>[4x]MQWSGARALEALLTVAGELRGPPLQLDTGQLLKIAKRGGVTAVEAVHAWRNALTGAPLNLTPEQVVAIASHDGGKQALETVQRLLPVLCQAHGLTPQQVVAIASHDGGKQALETVQRLLPVLCQAHGL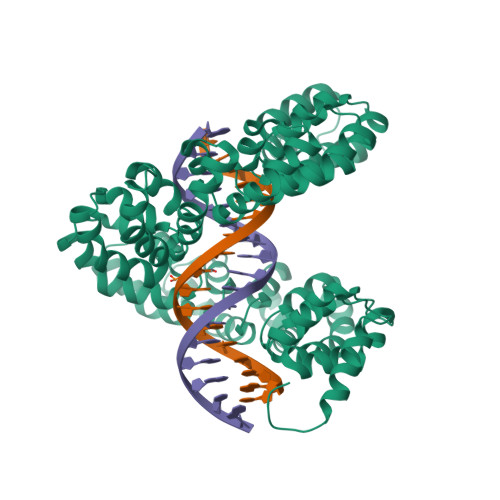TPEQVVAIASHDGGKQALETVQALLPVLCQAHGLTPEQVVAIASNGGGKQALETVQRLLPVLCQAHGLTPQQVVAIASNGGGKQALETVQRLLPVLCQAHGLTPQQVVAIASRGGGKQALETVQRLLPVLCQAHGLTPQQVVAIASNNGGKQALETVQRLLPVLCQAHGLTPQQVVAIASHDGGKQALETVQRLLPVLCQAHGLTPQQVVAIASNNGGKQALETVQRLLPVLCQAHGLTPEQVVAIASNGGGKQALETVQRLLPVLCQAHGLTPEQVVAIASHDGGKQALETVQRLLPVLCQAHGLTPQQVVAIASNGGGRPALESIVAQLSRPDPALAALTNDHLVALACLGGRPALDAVKKLEHHHHHH>[2x]GSVAGRIVIDDVQPVVSNGRYPAKAVVGEVVPVAATVWREGHDAVAATLVVRYHGTTYPDLADPPPGVPGADRTAVPIGDVMTPAAPVKPQRLPMSPGHTPDVFHGHFTPDRVGLWTYRVDGWGDPIASWRHNVTAKLDAGQGESELNNDLLVGARLLERAATGVPRELREALLEAAAALRAPGDPFTRAGAALSAEVSDLLAEYPLREFVTRGEQYGVWVDRPEARFSSWYEMFPRSTGGWDAEGRPVHGTFATAAEALPRIARMGFDVVYLPPIHPIGKVHRKGRNNSVTAAPGDVGSPWAIGSDEGGHDAVHPQLGTIEDFDEFVASARDLGLEVALDLALQCAPDHPWAREHPEWFTVLPDGSIAYAENPPKKYQDIYPLNFDNDPAGIYQEVLRVVRFWISHGVNIFRVDNPHTKPPNFWAWLIGQIKNENPDVLFLSEAFTRPARLYGLAKLGFTQSYTYFTWR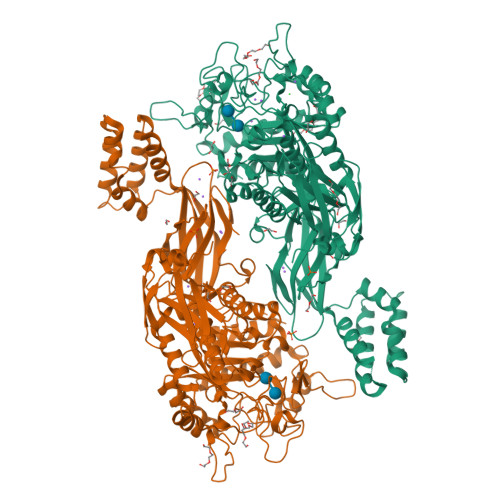TSKWELTEFGQEIAAKADIARPNLFVNTPDILHESLQHGGPGMFAIRAVLAATMGPAWGVYSGYELFENQPVRPGSEEYLNSEKYELRPRDFESALARGESLEPFLTRLNEIRRLHPALRELRTIRFHHVDNDALLAYSKFDPGTGDTVLVVVTLNPFGAEEATLWLDMPELGMEPYDRFWVRDEITGEEYQWGQANYVRLDPAKAVAHVLNMPLIPADKRLQLLRRE> MASVDFKTYVDQACRAAEEFVNVYYTTMDKRRRLLSRLYMGTATLVWNGNAVSGQESLSEFFEMLPSSEFQISVVDCQPVHDEATPSQTTVLVVICGSVKFEGNKQRDFNQNFILTAQASPSNTVW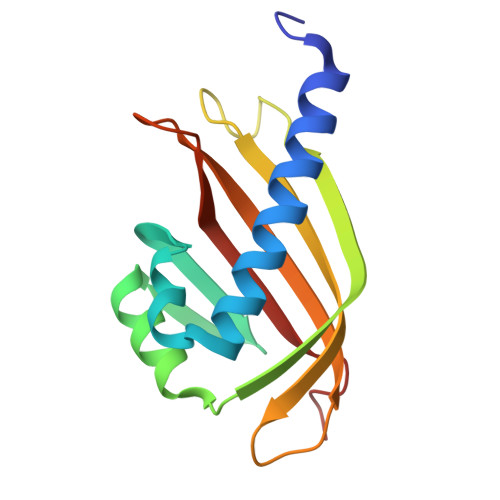KIASDCFRFQDWAS> MRGSHHHHHHGSMYLDSQLAERRSMHGVLVDIYGLGVLITGDSGVGKSETALELVQRGHRLIADDRVDVYQQDEQTIVGAAPPILSHLLEIRGLGIIDVMNLFGAGAVREDTTISLIVHLENWTPDKTFDRLGSGEQTQLIFDVPVPKITVPVKVGRNLAIIIEVAAMNFRAKSMGYDATKTFEKNLNHLIEHNEETD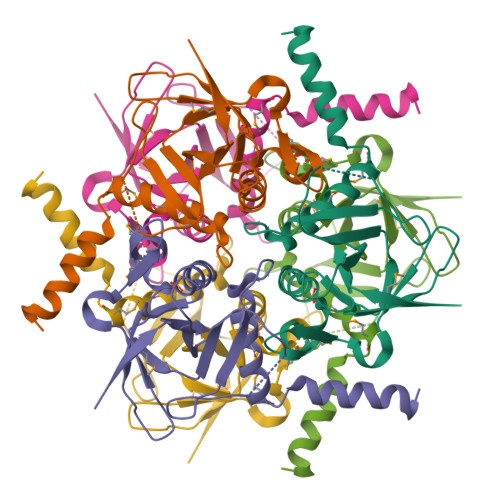QNSSGDK>MSTTQTPDLDAIVIGAGFGGIYMLHKLRNDLGLSVRVFEKGGGVGGTWYWNKYPGAKSDTEGFVYRYSFDKELLREYDWTTRYLDQPDVLAYLEHVVERYDLARDIQLNTEVTDAIFDEETELWRVTTAGGETLTARFLVTALGLLSRSNIPDIPGRDSFAGRLVHTNAWPEDLDITGKRVGVIGTGSTGTQFIVAAAKMAEQLT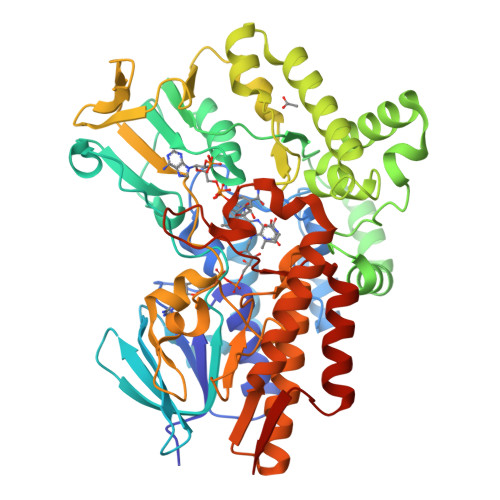VFQRTPQYCVPSGNGPMDPDEVARIKQNFDSIWDQVRSSTVAFGFEESTVEAMSVSESERQRVFQQAWDKGNGFRFMFGTFCDIATNPEANAAAAAFIRSKIAEIVKDPETARKLTPTDLYAKRPLCNEGYYETYNRDNVSLVSLKETPIEEIVPQGVRTSDGVVHELDVLVFATGFDAVDGNYRAMNLRGRDGRHINEHWTEGPTSYLGVTKAGFPNMFMILGPNGPFTNLPPSIEAQVEWISDLIDKATREGLTTVEPTADAEREWTETCAEIANMTLFPKADSWIFGANIPGKRHAVMFYLGGLGNYRRQLADVADGGYRGFQLRGERAQAVA[2x]>[20x]SSD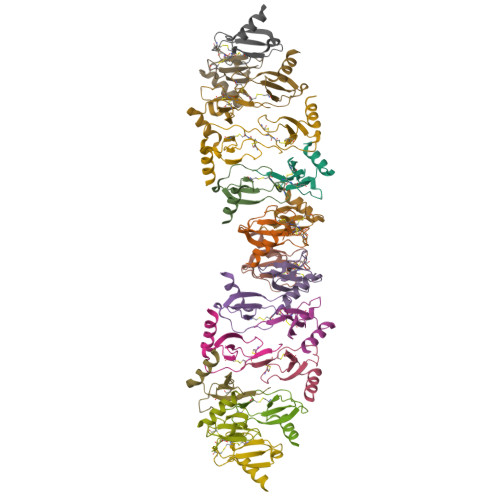TTPCCFAYIARPLPRAHIKEYFYTSGKCSNPAVVFVTRKNRQVCANPEKKWVREYINSLEMS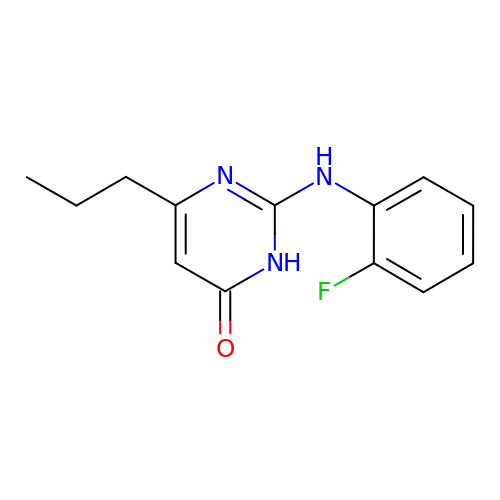2-[(2-fluorophenyl)amino]-6-propylpyrimidin-4(3H)-one | C13 H14 F N3 O | PKDFHRREPYQILX-UHFFFAOYSA-N> MGSSHHHHHHSSGRENLYFQGMIKEMIEDFISKGGLIFTHSGRYTNTNNSCFIFNKNDIGVDTKVDMYTPKSAGIKNEEGENLWQVLNKANMFYRIYSGELGEELQYLLKSCCTAKEDVTTLPQIYFKNGEGYDILVPIGNAH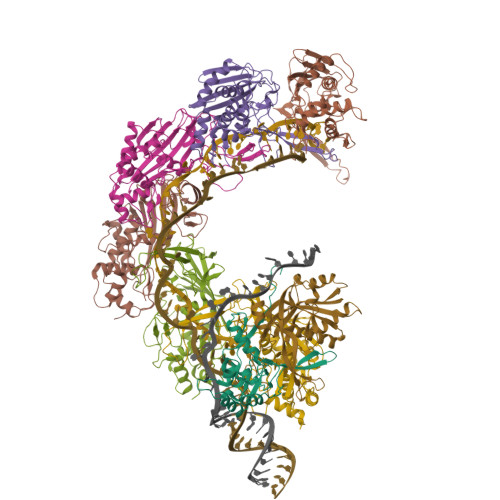NLISGTEYLWEHKYYNTFTQKLGGSNPQNCTHACNKMRGGFKQFNCTPPQVEDNYNA;> MGSSHHHHHHSSGRENLYFQGMRKFIIVKNVKVDGINAKSSDITVGMPPATTFCGLGETMSIKTGIVVKAVSYGSVKFEVRGSRFNTSVTKFAWQDRGNGGKANNNSPIQPKPLADGVFTLCFEVEWEDCAEVLVDKVTNFINTARIAGGTIASFNKPFVKVAKDAEELASVKNAMMPCYVVVDCGVEVNIFEDAVNRKLQPMVNGYKKLEKIVDNKHMRDKFTPAYLATPTYTMIGYKMVSNVDNFDQALWQYGENTKVKTIGGIYND;>[6x]MGSSHHHHHHSSGRENLYFQGMTKLKAPAVLAYSRKINPTNALMFAVNWSDRDNTTAVMVGTKTVAGTQSVRGNPNDADKGNIQTVNFANLPHNKNTLLVKYNVKFVGDVFKAELGGGEYSNTLQTALENTDFGTLAYRYVYNIAAGRTLWRNRVGAESIETVITVNDQTFTFSDLLVNEFDEDVDVAEIADMVAGVLSGEGFVTLKVEHYMLLGEGSEVFPSQEFVENSKLSKQLFDLNGQAAMHDQKIGNAIRTIDTWYEDATTPIAVEPYGSVVRNGVAYRAGNKTDLFTLMDGAVNGKSLTEEDQMFVTANLIRGGVFGGGKD> GSAAASPAWMPAYACQRPTPLTHHNTGLSEALEILAEAAGFEGSEGRLLTFCRAASVLKALPSPVTTLSQLQGLPHFGEHSSRVVQELLEHGV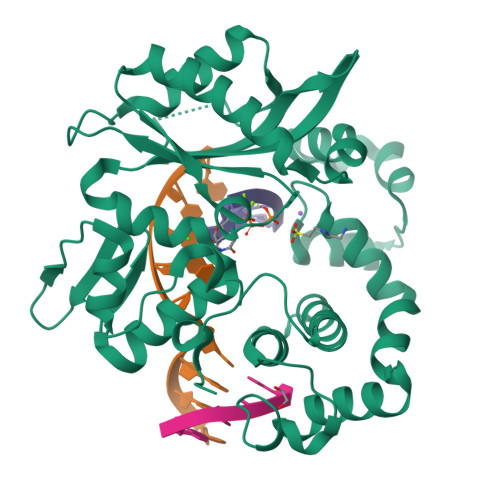CEEVERVRRSERYQTMKLFTQIFGVGVKTADRWYREGLRTLDDLREQPQKLTQQQKAGLQHHQDLSTPVLRSDVDALQQVVEEAVGQALPGATVTLTGGFRRGKLQGHDVDFLITHPKEGQEAGLLPRVMCRLQDQGLILYHQHQHSCCESPTRLAQQSHMDAFERSFCIFRLPQPGSWKAVRVDLVVAPVSQFPFALLAWTGSKLFQRELRRFSRKEKGLWLNSHGLFDPEQKTFFQAASEEDIFRHLGLEYLPPEQRNA>MRSRRVDVMDVMNRLILAMDLMNRDDALRVTGEVREYIDTVKIGYPLVLSEGMDIIAEFRKRFGCRIIADFKVADIPETNEKICRATFKAGADAIIVHGFPGADSVRACLNVAEEMGREVFLLTEMSHPGAEMFIQGAADEIARMG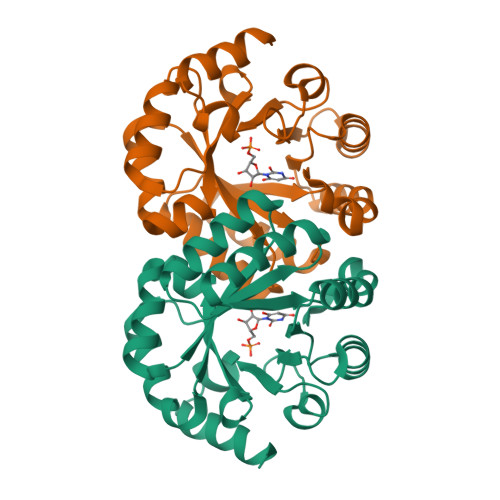VDLGVKNYVGPSTRPERLSRLREIIGQDSFLISPGAGAQGGDPGETLRFADAIIVGRSIYLADNPAAAAAGAIESIKDLLNP[2x]> MSKTRRWVIILLSLVALILIGVNLADRDDTQTEVINNNDPTYKSDHSDTVVYSPEGALNYRLIAQHVEYFSDDGISWFTQPVMTTFDKDKVPTWSIKSDRAKLTNDRMLYLYGHVEVNALTADSQLRKITTDNAQI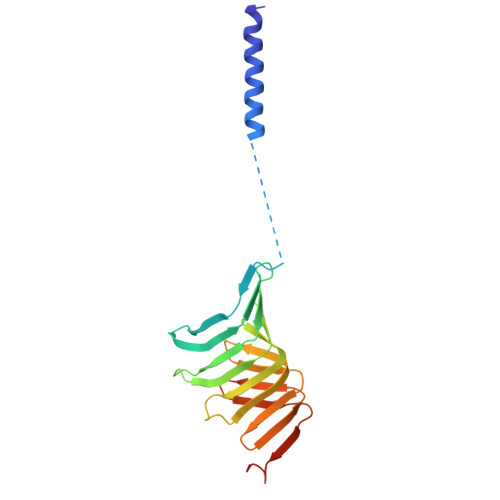NLVTQDVTSQDLVTLYGTTFNSSGLRMRGNLRSKNAELIEKVRTSYEIQNKQTQPLVPR In contrast, both cyclic nucleotides mediate transcription activation by Sinorhizobium meliloti Clr, mapping to cluster G of Crp-like proteins. We present crystal structures of Clr-cAMP and Clr-cGMP bound to the core motif of the palindromic Clr DNA binding site (CBS). The structures show a Clr dimer that is bound to CBS-DNA. The individual subunits fold into two domains linked by helix α5 (residues P123 to L149), which is the Clr dimerization interface.

The cNMP binding site located in the N-terminal domain is stoichiometrically occupied by cAMP and cGMP, respectively. The binding modes of the phosphate and sugar moieties are identical, involving G85 and E86 within α4 as well as R95 and S96 of the following loop. The side chain of S96 is flipped toward the phosphate only in the cGMP-bound complex. The nucleobase of cGMP is flipped to the syn conformation, while it occupies the anti conformation in the Clr-cAMP complex. While cAMP interacts via its primary N6-amine with both T140 and T141, cGMP forms hydrogen bonds between T140 and its C-6 carbonyl group as well as between T141 and the N2-amine. The latter interaction between the N2-amine of cGMP and T141 of the adjacent molecule is a substantial difference between Clr and the inactive cGMP complex of E. coli CAP. As cGMP is bound in a syn conformation, the interactions can be retained. In contrast to any previous findings in E. coli, we clearly established that Clr performs an identical binding movement via a 140TT motif for both cNMPs. In contrast, cGMP binding by Clr alone proceeds endothermically and with apparently lower affinity (KD, ~24 μM). Compared to the Clr–cAMP–CBS-DNA complex, ternary complex formation with cGMP gives similar affinities and also relies on both contributions.

>[2x]MAEVIRSSAFWRSFPIFEEFDSETLCELSGIASYRKWSAGTVIFQRGDQGDYMIVVVSGRIKLSLFTPQGRELMLRQHEAGALFGEMALLDGQPRSADATAVTAAEGYVIGKKDFLALITQRPKTAEAVIRFLCAQLRDTTDRLETIALYDLNARVARFFLATLRQIHGSEMPQSANLRLTLSQTDIASILGASRPKVNRAILSLEESGAIKRADGIICCNVGRLLSIADPEEDLEHHHHHHHH> ETGELKIECPHTIGLGQGLVIGSVELPPVPLTQVESLKLESSCNFDLHTSTSSQQPFTKWTWEMKSDLAENTQASSTSFQTKSSEINLRGLCLVPPLVIETAARTRKTIACFDLSCNQTACQPTVFLIGPIQTCITTKSCLLGLGDQRIQVNYEKTYCVSGQLVEGVCFNPVHTMALSQPSHTYDIVTVMVRCFLIAKKVSTGDSMKLEKSFETLVQKTSCTGNGFQ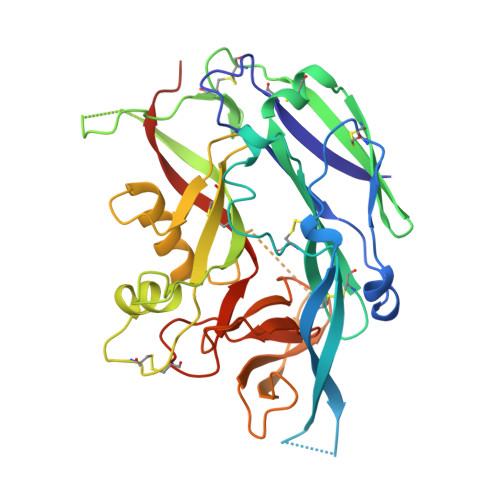GYYICLVGSSSEPLYIPTLDDYRSAEVLSRMAFAPHGEDHDVEKNAISAMRIIGKVTGKAPSTESSDTIQGVAFSGNPLYTSTGVLTAKDDPVYIWAPGIIMEGNHSVCDKKTLPLTWTGFIPLPGEIEKTGTKHHHHHH> MKHRIEYAITNAVFVKADELSYLSFRVSGKVIEVYKDLGDYVKRGEALAKLDPTYYELEKRTLEKKMSALLEKKKALEIKIQKLEKGLHISLSAKKLKVESLKKKREALREKLLQVEEKIKLVKLDWERYKSLFQKGLIPRRKFEEVDTNLKVLLHEREYLEKSIQEINTEIKRAKKGIENARNEFKTIEELKKELSSLEEEIKSLKERIKTAEQKIKDTVLIAPFDGVVAKRFISRGDVVRAGQPAFALVNPESFYVEVLLEETK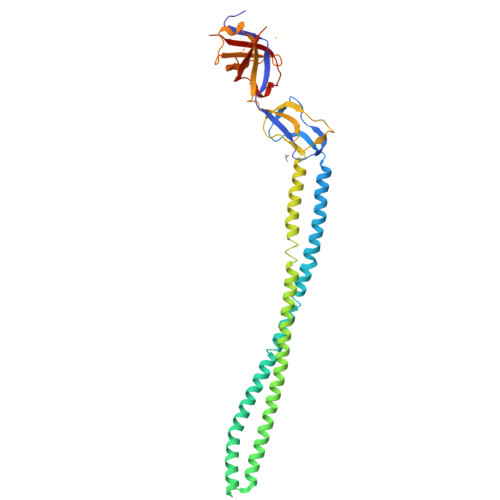LKGVKVGNKAYVRLDAYPDILFEGVVEEISPASAATFALVPRDVSAGEFTKVVQRIPVKIKITKGDLSLLRVGMGGEVEIRRTRLEHHHHHH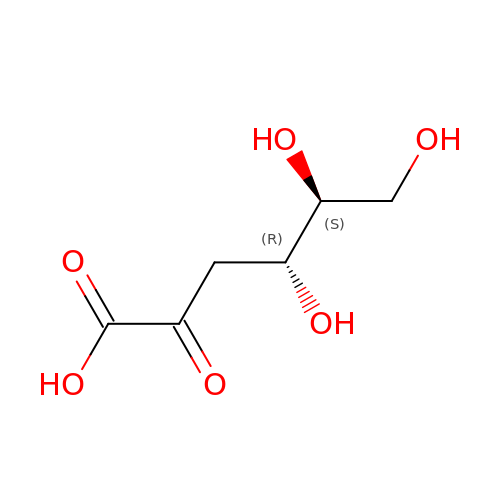L-2-keto-3deoxy-gluconate | C6 H10 O6 | WPAMZTWLKIDIOP-WUJLRWPWSA-N> MSSTEVFGALAPVGRTEVADALSSHANSKDARSLRYEPYANRLIKLQTAMVPPKVDGTSERVAEVVKGLAEQGAIYPDQMGAIHSDLLNRVYTWNS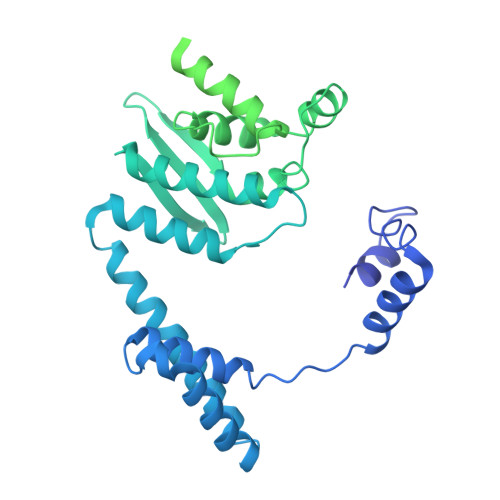MGVQESIQALVNDVIHGQNKVLQDELARTREIANASMLTRFFDSLYKTVDRGQRNFEGFKKLLRLFVNNVPNAEVYSSGGSFSLQINMGGQSQNINLTNAFDNLKDIWGARWDAVNNPRIGALLTPNTRALLFFVSTFYDYGSMEPGSYLDNLMRLYKEAIRADTDAEGDAIMELGDAGANLNLKFNQYKDTLNYLLQNKPSVPQTGPLEMSPEQESLFKYLMRQLRRALKDGVNSDIAISTMAQYVDPRLYTSNKVFIDKLQNYLLMASARNPYYYKTIVLDPHWVPPAGLYTDNFVIPEMMPNFSDFASELEYGGPSRDEYFDDSPFRPPPQKKFTEKEQADYDSLINFFDSTLGVQSEAGWIADHRLPQAFDGALNVSERTPYNTPLPDDAPMRSRNASVSSATDALGQLKLSGTGGAGFFDSLKPSVGTRRSTGLAKGLAGTGQPPCPWPASVGYASAGYGPARGIRGSGLARRALAARGLRQGKRLRFY>YVEFATKRGSPNPTRAAAVKAAFQTSWNAYHHFAFPHDDLHPVSNSFDDERNGWGSSAIDGLDTAILMGDADIVNTILQYVPQINFTTTAVANQGSSVFETNIRYLGGLLSAYDLLRGPFSSLATNQTLVNSLLRQAQTLANGLKVAFTTPSGVPDPTVFFNPTVRRSGASSNNVAEIGSLVLEWTRLSDLTGNPQYAQLAQKGESYLLNPKGSPEAWPGLIGTFVSTSNGTFQDSSGSWSGLMDSFYEYLIKMYLYDPVAFAHYKDRWVLGADSTIGHLGSHPSTRKDLTFLSSYNGQSTSPNSGHLASFGGGNFILGGI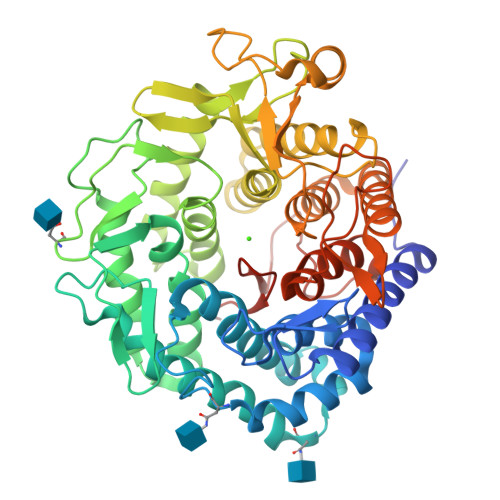LLNEQKYIDFGIKLASSYFGTYTQTASGIGPEGFAWVDSVTGAGGSPPSSQSGFYSSAGFWVTAPYYILRPETLESLYYAYRVTGDSKWQDLAWEALSAIEDACRAGSAYSSINDVTQANGGGASDDMESFWFAEALKYAYLIFAEESDVQVQATGGNKFVFNTEAHPFSIRSSSRRGGHLA[4x]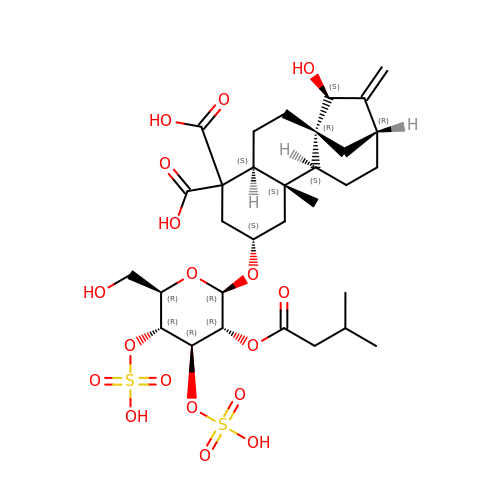Carboxyatractyloside | C31 H46 O18 S2 | AQFATIOBERWBDY-LNQSNDDKSA-N> SASKQF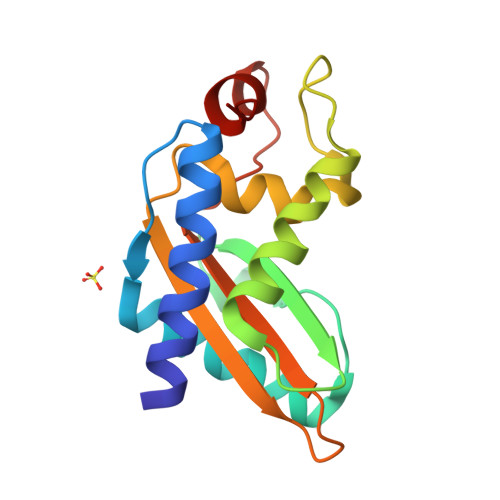HNEVLKAHNEYRQKHGVPPLKLCKDLNREAQQYSEALASTRILKASPESSRGQCGENLAWASYDQTGKEVADRWYSAIKNYNFQQPGFTSGTKAFTAMVWKNTKKMGVGKASASDGSSFVVARYFPAGGVVNEGFFEENVLPPK(10S,13R)-3-{2-[{2-[bis(carboxymethyl)amino]ethyl}(carboxymethyl)amino]ethyl}-10-hydroxy-5,16-dioxo-13-(tetradecanoyloxy)-9,11,15-trioxa-3,6-diaza-10-phosphanonacosan-1-oic acid 10-oxide | C47 H87 N4 O17 P | 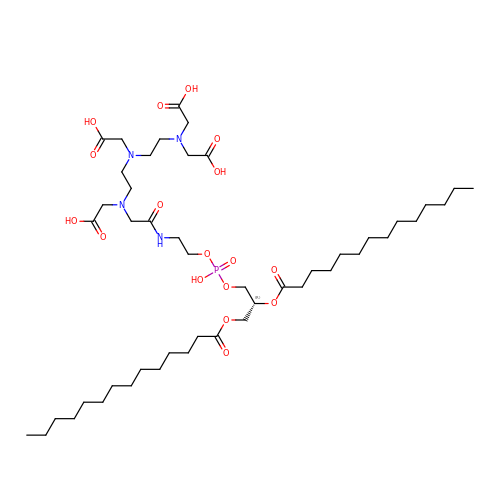DAAFWSGIXJNAQE-RRHRGVEJSA-N> MLHFTSLFRARAIIKRRTPQLWGAPGAPIIRMRGHHVVWKFQSYDLFVEHTHKRRNSDARLLHYLGKHCPHPQKSLWSPDTPVAQDRHLFMLTTVDVDAFKYWFGVKRCRLSMRPWALLAKAGLLPP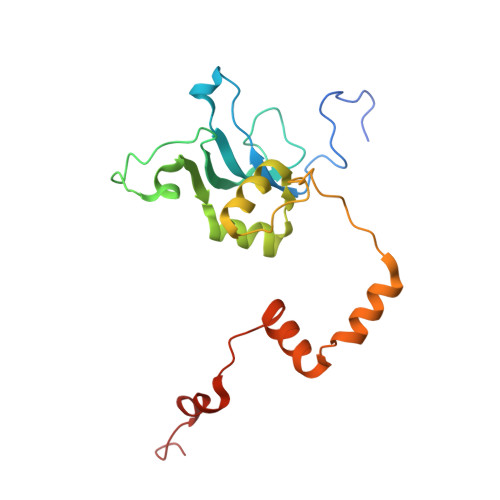SLRQNSKIMPKPIFDKEQLMRYYLANRKEEATIEREDYLNYKNSLVKSEEERAAERPVAPYL> MPKLVTWMNNQRVGELTKLANGAHTFKYAPEWLASRYARPLSLSLPLQRGNITSDAVFNFFDNLLPDSPIVRDRIVKRYHAKSRQPFDLLSEIGRDSVGAVTLIPEDETVTHPIMAWEKLTEARLEEVLTAYKADIPLGMIREENDFRISVAGAQEKTALLRIGNDWCIPKGITPTTHIIKLPIGEIRQPNATLDLSQSVDNEYYCLLLAKELGLNVPDAEIIKAGNVRALAVERFDRRWNARRTVLLRLPQEDMCQTFGLPS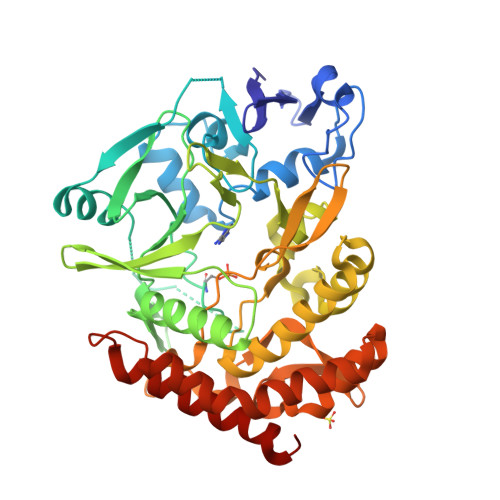SVKYESDGGPGIARIMAFLMGSSEALKDRYDFMKFQVFQWLIGATDGHAKNFSVFIQAGGSYRLTPFYDIISAFPVLGGTGIHISDLKLAMGLNASKGKKTAIDKIYPRHFLATAKVLRFPEVQMHEILSDFARMIPAALDNVKTSLPTDFPENVVTAVESNVLRLHGRLSREYGSK> ATFEIVNRCSYTVWAAASKGDAALDAGGRQLNSGESWTINVEPGTKGGKIWARTDCYFDDSGRGICRTGDCGGLLQCKRFGRPPTTLAEFSLNQYGKDYIDISNIKGFNVPMDFSPTTRGCRGVRCAADIVGQCPAKLKAPGGGCNDACTVFQTSEYCCTTGKCGPTEYSRFFKRLCPDAFSYVLDKPTTVTCPGSSN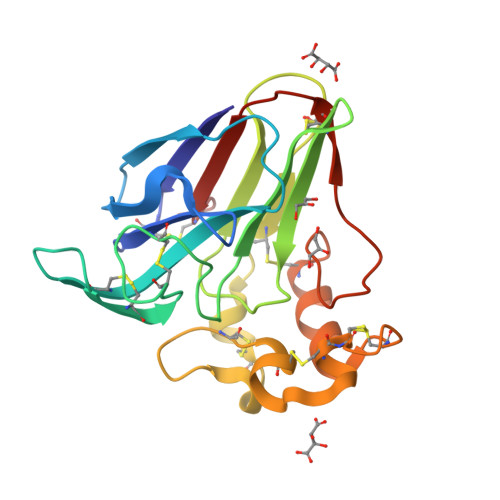YRVTFCPTA Com is a small zinc finger protein that regulates the translation of bacteriophage Mu Mom RNA. The regulation occurs via Mom RNA binding and structural rearrangements leading to an exposition of translation start site. We attempted to co-crystallize Com with its natural RNA target, as well as with its variants designed computationally to form either a monomeric hairpin-loop structure or a homo-duplex form. Thus far, we obtained crystals and solved the structure of an RNA homo-duplex form.

The 19-mer self-complementary RNA II duplex folds into a double helix of the A-form (A-RNA). The RNA duplex consists of 14 canonical Watson-Crick base pairs (A-U, C-G) and 5 non-canonical base pairs (four A•C and one G•G pair in the middle of the duplex). All non-canonical base pairs form two hydrogen bonds. The central G•G base pair, although showing static disorder, breaks the chemical and crystallographic symmetry of the helix. This non-canonical pair was modeled as two alternative conformations: one with syn-anti and other with the anti-syn orientation of base rings. The Cl- anion is located on the opposite side of the RNA helix, minor groove, and bound to G11 of chain A. In general, the presence of non-canonical base pairs G•G and C•A does not distort the A-RNA form of RNA II, and the overall structure is stable, with the characteristic 11 base pairs per turn, the C3' endo conformation of the sugar rings, and the presence of the axial hole. The occurrence of double hydrogen bonding for the A•C pair is likely due to protonation of the adenine, on nitrogen in position 1, which can be promoted in the acidic crystallization condition (pH 4.6), but we cannot rule out that one of the bases is present as an imino tautomer, thus allowing two hydrogen bonds to be formed. In RNA II, the G residue of the GA dinucleotide is involved in canonical base pairing. This situation may reduce the accessibility of the RNA II sequence motif for interaction with Com, which prefers the GA dinucleotide to be available in a flexible, single-stranded form (as indicated by high reactivity of GA dinucleotides at the beginning of each strand in SHAPE probing).

>[2x]AGAGAACCCGGAGUUCCCU Most forms of damage to the heterocyclic nucleobases of DNA are repaired by mechanistically related pathways collectively referred to as the base-excision repair (BER) mechanism. Both the recognition of damaged sites and initiation of repair by BER are performed by DNA glycosylases, lesion-specific enzymes that recognize specific nucleobase damages in the genome and catalyze their excision through cleavage of the glycosidic bond. Among them, 8-oxoguanine (oxoG, OG) presents the greatest challenge to the DNA glycosylases responsible for its repair, due to its unique combination of structural innocuousness, extrordinary mutagenicity, and chronic low-level production. The question addressed here is whether the 8-oxoguanine DNA glycosylase responsible for oxoG recognition and repair in humans, namely hOGG1, interrogates DNA in the same way as the functionally equivalent bacterial enzyme MutM, despite the lack of an overall structural and sequence similarity between these two oxoG repair enzymes. In summary, we present X-ray crystallographic structures of human DNA glycosylase hOGG1 interrogating DNA lesions in their intrahelical position, achieved by covalent trapping of an ordinarily transient state in DNA recognition.

On the basis of this screen, we have selected the Y207C variant, because it crosslinks efficiently but is substantially distant from the active site of the enzyme to participate in the catalysis and does not interact with DNA in native LRC, and crosslinked it through the X8 linker to the minor groove N2-exocyclic amine of 3′ guanine of the target nucleobase. The complex produced a crystal structure at 2.35 Å resolution with an intrahelical target G•C base-pair, hereafter referred to as the interrogation complex (IC). In both IC and EC structures, the target G•C and oxoG•C base-pairs are unambiguously intrahelical, with a root-mean-square deviation (RMSD) of 0.244 Å between the two structures, in which the RMSD superposition was performed for all atoms. In both structures, the target strand remains in the same position with respect to hOGG1, but the non-target DNA strand of the IC structure has translocated by half a nucleotide step toward the 3′ end of the non-target strand, marked with an arrow. For example, R154 and R204 contact the non-target strand backbone, instead of interacting with the C opposite to oxoG (i.e., the estranged C in LRC). In addition, Y203 does not invade the helical stack and remains at the periphery of the minor-groove face of DNA. Similarly, N149 rests on the minor-groove face of the target G•C (in IC)/oxoG•C base-pair (in EC) and hydrogen bonds with both bases. In the presence of oxoG, hOGG1 establishes a stable contact with the target strand, while in the case of G it fluctuates back-and-forth. Consistent with this, the target strand with oxoG shows smaller root-mean-square fluctuation (RMSF) of atomic position than that with G.

> GSEGHRTLASTPALWASIPCPRSELRLDLVLPSGQSFRWREQSPAHWSGVLADQVWTLTQTEEQLHCTVYRGDKSQASRPTPDELEAVRKYFQLDVTLAQLYHHWGSVDSHFQQVAQKFQGVRLLRQDPIECLFSFICSSNNNIARITGMVERLCQAFGPRLIQLDDVTYHGFPSLQALAGPEVEAHLRKLGLGYRARCVSASARAILEEQGGLAWLQQLRESSYEEAHKALCILPGVGTKVADCICLMALDKPQAVPVDVHMWHIAQRDYSWHPTTSQAKGPSPQTNKELGNFFRSLWGPYAGWAQAVLFSADL OXIDIZED GLUTATHIONE DISULFIDE | C20 H32 N6 O12 S2 | 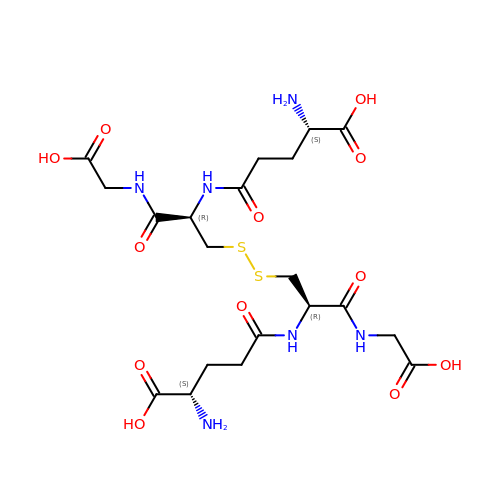YPZRWBKMTBYPTK-BJDJZHNGSA-N> KETA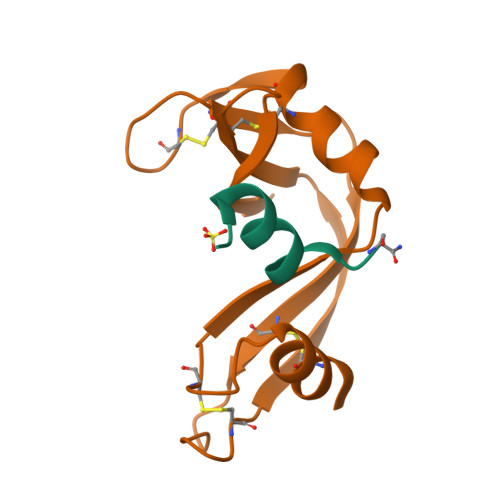AAKAERQHMDS;> NYCNQMMKSRNLTKDRCKPVNTFVHESLADVQAVCSQKNVACKNGQTNCYQSYSTMSITDCRETGSSKYPNCAYKTTQANKHIIVACEGNPYVPVHFDASV>MASKKENLKSLFSNTRTRVIIIFTAALLIIAVVIGFFKIRGATTGSIAAAEVSTVPGGIQSIPGVLDPTAQYAKLQEEQNITQAQVAEKTGGSAIPTIIRTQALGEGVGVIGSQSGVGFAALAQEELGGPQRSLWIQELQDGSCSKSVITKVVNQGAQLTDLKAACSCVQLKDSGYGLQELEQVCECKELKSAGYNARQLKEAGYSAGRLRNCGFDACELRNAGFTAQEMKDGGFSDGELKGAGFSDAEIAKASGLPDGITADDVRKAGCGAAALAKLRQAGVSASAIRKISGCTAEQLKAAGYTAKELKDAGFSAADLRRAGFSAAELKDAGFTARDLLNAGFTPADLAKAGFSDAQIKAAQAELPPGITPQDVKNAGCDVEALKKEREAGVSAALIRQYAGCSAQALKAAGFTDADLANAGFTPAQISAATPLSDAEIKAAGCDPDKLKKLFSAGVSAKRIKELNGCSAEALKAAGYDAQSLLAAGFTPQELLAAGFTPKQLEDAGLNPVSIIADGRVADCSVESLKKARAAGVSALTIKQTLGCSAAALKAAGYTAKELKDAGFTAAELKAAGFSAKELKDAGFTAKELRDAGFSAQELKDVGFSAKDLKDAGFSAAELKAAGFTAAQLKAAGFSAKDLKDAGFSAAELKAAGFSAKELK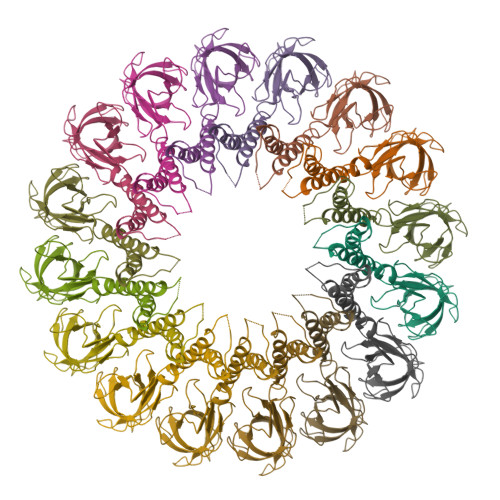DAGFSASDLKNAGFSAKELKDAGFSASDLKSAGFSASELKNAGYSADELKKAGYTSAELRNAGFSPQESAVAGLQGPDLQQLDSSITGIPSIPGATPRPTTSDAASSAEQLQAILQKQNEQLAEQKYQQEIQQRTSDMLTAATQLVQDWKQVETQVYTEGTEETKTSGGESAVPGTGTGTGSNNQPVDQGAVSAQNQAIIKTGDIMFAVLDTSVNSDEPGPILATIVTGKLKGSKLIGSFNLPSNADKMVITFNTMSIPGAEKTISISAYAIDPNTARTALASRTNHHYLMRYGSLFASSFLQGFGNAFQSANTTITIGGTGGGNNITVANGVRRSTLENAVIGLATVGKAWSQQAQQLFNTPTTVEVYSGTGLGILFTQDVTTI[16x]> QQQKPQRRP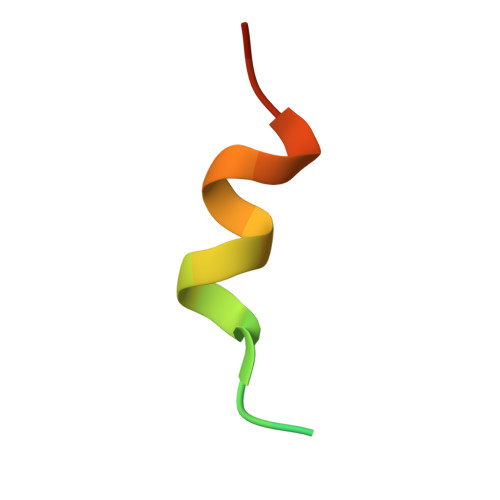CSELLKYLTTNDD>MALILTFLGKSGVARTKIAIAAAKLLASQGKRVLLAGLAEPVLPLLLEQTLTPDPQQIAPNLEVVQFQSSVLLERNWEEVKKLEAQYLRTPIIKEVYGQELVVLPGMDSALALNAIREYDASGKYDTIVYDGTGDAFTLRMLGLPESLSWYVRRFRQLFVNSDLGKTIAESPLIQPLISSFFNVNWTADNFAQPTNQVNNFLDKGKEALADPKRVAAFLVTTADPLEVVSVRYLWGSAQQIGLTIGGVIQVSSQT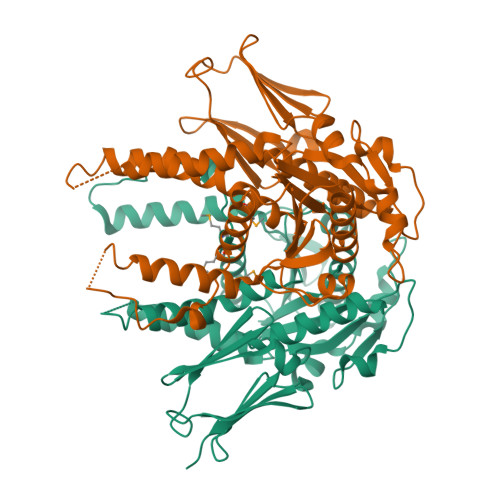EGDLSAEFTPLSVTVVPDVTKGDWQPLIDALPNFVEQAEQAPKPITIDTHNRQVRLFLPGFDKKQVKLTQYGPEVTVEAGDQRRNIFLPPALSGRPITGAKFQNNYLIISFLEHHHHHH[2x]BETA-6-HYDROXY-1,4,5,6-TETRHYDRONICOTINAMIDE ADENINE DINUCLEOTIDE 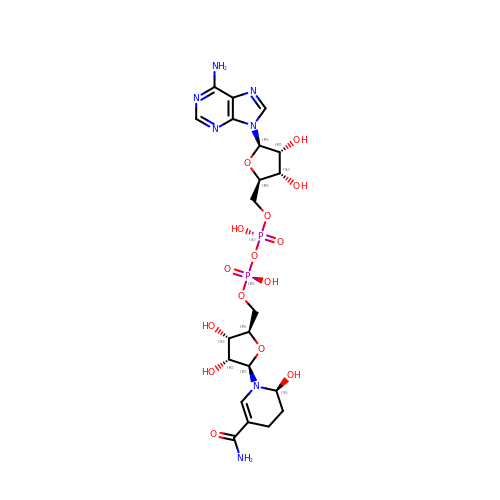| C21 H31 N7 O15 P2 | IDBZKGQRLBFUFQ-VPHRTNKSSA-N>[4x]MVQKWMQRMIIVDNNKLNVRALPSFIDYFNGIYGFATGIKDIMGMIFKTDTGGSNLTLDEILKNQNLLNDISGKLDGINGDLGDLIAQGNLNSELAKELLKISNEQNQMLNHVNAQLNAINSTLNIYLPKITSMLNEVMKQNHVLSLQIEFLSKQLQEISDKLDIINLNVLINSTLTEITPAYQRIKYVNEKFDELTSTVEKNPKSYQDNVTKEVIENLNELTELAKSVTKNDMDSFEFYLQTFHDVMTGNNLFGRSALKTASELITKENVTTRGSEIGKVYNFLIVLTSLQAKAFLTLTACRKLLGLTDIDYTQIMNHHIDGQKREFRINILPTLSNNFSNPSYSKNRGSDIDDPIVVLEAAPGYALIGFEILNDPLPILKGYQARLKPNYQVDRESMSETIYGDIHKLFCPKQLEQKYYIKDIEFPEGYVITKIVFEKRLNQLGYEVTANFYDPSTGSIDLNKVKVESWKEKSCEEDSCEDEYSIIKAETDGIYMPLGVVSETFLTPIYGFGLTVDEKNQKITLTGKSYLRESLLETDLLNNETYLIASPDGYISSIVENWNITSDNTGSWRANNNNAFVDKADTIKGSSSLYTHKDGEFSQFIGNKLKPKTNYVIQYVIKGRPAIYLKNNKDTLFEDTKNNFSDFQTVTKKFNSGVNPSEIYFLFKNQSEYEAWGNNFIILEIKSLEFLPQMLKPEDWIPSGNVQMKDGGRLEILGDGYFKQFIKLENDSTYHLRLSVKGTGRVSIIDESKYLLFVNVKDEDLTRVIKNTSSKGECFIALEGTYVENSSTIFSNVSIVKE

The Vip3 (vegetative insecticidal protein 3) family proteins from Bacillus thuringiensis convey toxicity to species within the Lepidoptera, and have wide potential applications in commercial agriculture. The Vip3 proteins have molecular masses of ~90 kDa, and are secreted as soluble proteins that form tetramers in solution. They can be proteolytically processed by trypsin or insect gut extracts to yield products of ~65 kDa and ~21 kDa that remain closely associated in solution. Vip3 proteins are proposed to exert their insecticidal activity through pore formation, though to date there is no mechanistic description of how this occurs on the membrane.

We first examined the structure of the wild type, full length Vip3Bc1 by single particle cryoEM. The 3D reconstruction of the tetrameric assembly of Vip3Bc1 with a global resolution of 3.9 Å resolution was obtained (0.143 FSC threshold). Our Vip3Bc1 structure reveals a tetrameric assembly with C2 symmetry. Each tetramer comprises two dimers formed by conformationally distinct A:B monomers. Each monomer of Vip3Bc1 consists of 5 domains. Together, domain 1 and domain 2 form the N-terminal, largely alpha-helical portion of the protein. The two domains are connected by a contiguous alpha-helix (α3, residues 94-162) that interfaces with α2 (residues 61-88) undertaking a super-helical twist that gives the complex a distinct conical appearance. Domains 3-5 make up the C-terminal portion of the protein, primarily composed of β-strands. The interchain interactions that bring about the conical morphology and impart the C2 symmetry are formed at the interface between domains 1 and 2 on each of the monomers, with the rest of the complex not involved in oligomerisation.N-{2-[3-(piperazin-1-ylmethyl)imidazo[2,1-b][1,3]thiazol-6-yl]phenyl}quinoxaline-2-carboxamide 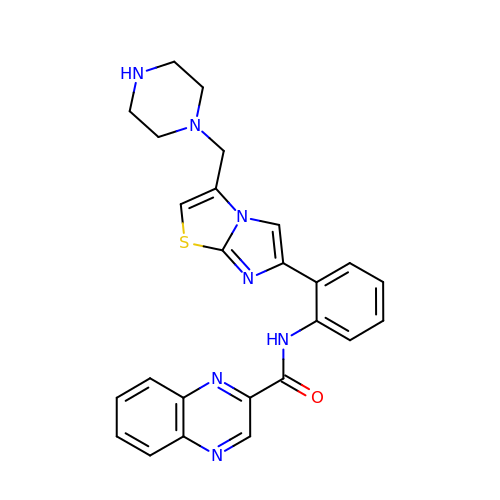| C25 H23 N7 O S | IASPBORHOMBZMY-UHFFFAOYSA-N>PLGSMSEEQVAQDTEEVFR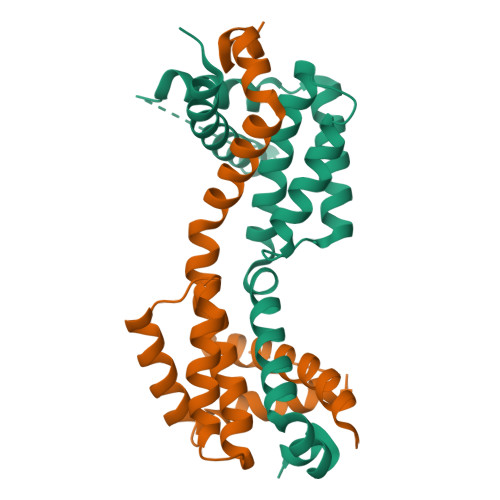SYVFYRHQQEQEAEGVAAPADPEMVTLPLQPSSTMGQVGRQLAIIGDDINRRYDSEFQTMLQHLQPTAENAYEYFTKIATSLFESGINWGRVVALLGFGYRLALHVYQHGLTGFLGQVTRFVVDFMLHHSIARWIAQRGGWVAALNLGNG[2x]>MSKAKIGIVTVSDRASAGIYEDISGKAIIDTLNDYLTSEWEPIYQVIPDEQDVIETTLIKMADEQDCCLIVTTGGTGPAKRDVTPEATEAVCDRMMPGFGELMRAESLKFVPTAILSRQTAGLRGDSLIVNLPGKPKSIRECLDAVFPAIPYCIDLMEGPYLECNEAVIKPFRPKAK[3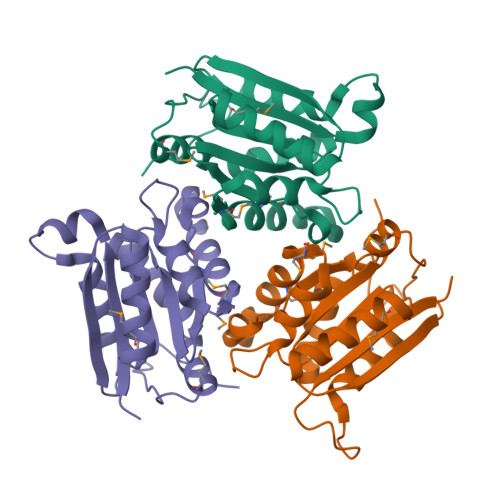x]>[4x]RSPWEENFSRSYPCDEKKQNDSVIAECSNRRLQEVPQTVGKYVTELDLSDNFITHITNESFQGLQNLTKINLNHNPNVQHQNGNPGIQSNGLNITDGAFLNLKNLRELLLEDNQLPQIPSGLPESLTELSLIQNNIYNITKEGISRLINLKNLYLAWNCYFNKVCEKTNIEDGVFETLTNLELLSLSFNSLSHVPPKLPSSLRKLFLSNTQIKYISEEDFKGLINLTLLDLSGNCPRCFNAPFPCVPCDGGASINIDRFAFQNLTQLRYLNLSSTSLRKINAAWFKNMPHLKVLDLEFNYLVGEIASGAFLTMLPRLEILD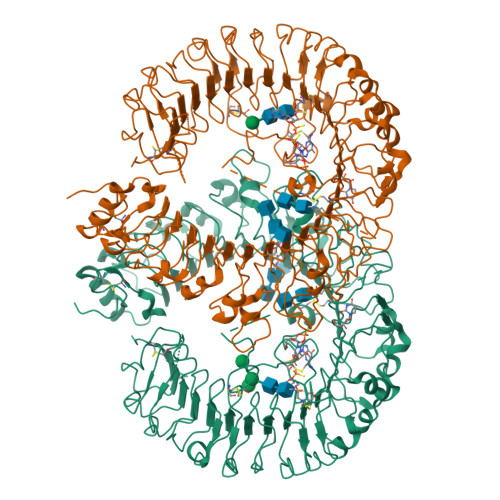LSFNYIKGSYPQHINISRNFSKLLSLRALHLRGYVFQELREDDFQPLMQLPNLSTINLGINFIKQIDFKLFQNFSNLEIIYLSENRISPLVKDTRQSYANSSSFQRHIRKRRSTDFEFDPHSNFYHFTRPLIKPQCAAYGKALDLSLNSIFFIGPNQFENLPDIACLNLSANSNAQVLSGTEFSAIPHVKYLDLTNNRLDFDNASALTELSDLEVLDLSYNSHYFRIAGVTHHLEFIQNFTNLKVLNLSHNNIYTLTDKYNLESKSLVELVFSGNRLDILWNDDDNRYISIFKGLKNLTRLDLSLNRLKHIPNEAFLNLPASLTELHINDNMLKFFNWTLLQQFPRLELLDLRGNKLLFLTDSLSDFTSSLRTLLLSHNRISHLPSGFLSEVSSLKHLDLSSNLLKTINKSALETKTTTKLSMLELHGNPFECTCDIGDFRRWMDEHLNVKIPRLVDVICASPGDQRGKSIVSLELTTCVSDVTEFLVPR Among them, the ubiquitin-like protein Atg8 (called LC3/GABARAP proteins in humans) plays a central role. In this study, we found that in both S. pombe and Saccharomyces cerevisiae, Atg8 physically interacts with Hfl1, a vacuole membrane protein. This interaction promotes the localization of Atg8 at the vacuole membrane in a lipidation-independent manner. hfl1Δ and atg8Δ caused the same vacuole-related phenotypes, which are not shared by other atg mutants. The structures showed that the Atg8-Hfl1 interaction is mediated by noncanonical mechanisms—using Hfl1 sequences adopting helical conformation (termed helical AIMs here) and in the case of budding yeast, involving a previously unreported binding site on Atg8.

To understand the atomic details of the SpHfl1-SpAtg8 interaction, we solved the crystal structure of SpAtg8 complexed with SpHfl1(386-409) at 2.2 Å resolution. The structure of SpAtg8 is similar to other Atg8-family proteins, consisting of a ubiquitin fold and two α-helices attached at the N-terminus. The structure of SpAtg8 can be superimposed on that of ScAtg8 with an rms difference of 0.8 Å for main-chain atoms except for those of terminal tails. As a result, the two AIM-binding hydrophobic pockets (W-site and L-site) on SpAtg8 resemble those on ScAtg8 and other Atg8 homologs. SpHfl1(386-409) is comprised of an extended coil followed by an α-helix, and interacts with the W-site, the L-site, as well as α3 of SpAtg8, burying ~2000 Å2 of surface area (detailed interactions are summarized in Figure 3—figure supplement 3A). SpHfl1(386-409) forms little interaction with crystallographically adjacent SpAtg8 molecules, suggesting that the complex structure is not markedly affected by crystal packing. Strikingly, SpHfl1(386-409) neither forms an intermolecular β-sheet with β2 of Atg8 (middle), nor uses two hydrophobic residues separated by two residues to engage the W-site and the L-site. Instead, SpHfl1(386-409) uses Phe388 at the coil and Tyr398 at the helix for binding to the W-site and the L-site, respectively, with as many as nine residues between them. In addition, a hydrophobic interaction is formed between Leu386 of SpHfl1 and a hydrophobic pocket near the W-site, some electrostatic interactions are formed between the side-chains of Asp391 and Glu395 of SpHfl1 and Lys46 and Arg28 of SpAtg8, respectively, and two hydrogen bonds are formed between the main-chain of SpHfl1 and the side-chain of SpAtg8. Alanine-substitution of SpHfl1 Phe388 (F388A) and Tyr398 (Y398A), which bind to the W-site and the L-site in SpAtg8, resulted in ~4 fold and ~1000 fold decrease in the affinity with SpAtg8, respectively. This result suggests that binding to the L-site is much more important than that to the W-site for the SpHfl1-SpAtg8 interaction, which is in contrast to the interactions between canonical AIMs and Atg8 where the W-site binding is usually more important than the L-site binding.

> GPHMRSQFKDDFSFEKRKTESQRIREKYPDRIPVICEKVDKSDIAAIDKKKYLVPSDLTVGQFVYVIRKRIKLSPEKAIFIFIDEILPPTAALMSTIYEEHKSEDGFLYITYSGENTFG;> MLQFEIDDEMEPLYNQAKQMRYGDYLEVLFQ>[2x]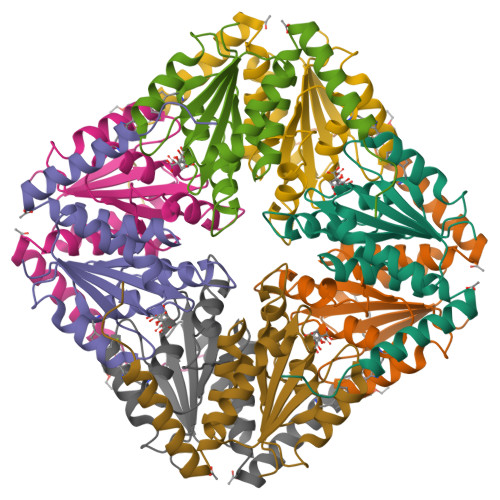MMSETAPLPSASSALEDKAASAPVVGIIMGSQSDFETMRHADALLTELEIPHETLIVSAHRTPDRLADYARTAAERGLNVIIAGAGGAAHLPGMCAAWTRLPVLGVPVESRALKGMDSLLSIVQMPGGVPVGTLAIGASGAKNAALLAASILALYNPALAARLETFRALQTASVPNSPITEDK> MGSSLMTEHKKRIDPVGAMLESKLLEAEFSPAVAAKLAALSQHYTPAELVRALPQSLANMLDNQGDDIVRQGGVVALVGPTGVGKTTSLAKLAARFAAHHGPEQVALITTDHYRIGAYEQLATYGKIMGCPVKQAHDLNELEQILYQFRNRKLVLIDTAGMGQRDMRLYQQLDNLTANSRIPIRSYLVLSATGQRRVLQDAVNHFKRIPLSGAVLTKLDESVSLAGALSVLIQSGLPLSYVTDGQRVPEDMKVADTLMLAQQALATLDSTEQQSLQDTAWSDNMACAFEHHHHHH

The GTPase FlhF, a signal recognition particle (SRP)-type enzyme, is pivotal for spatial–numerical control and bacterial flagella assembly across diverse species, including pathogens. FlhF, together with SRP54 (or Ffh) and FtsY, belongs to an evolutionarily conserved protein family with only three members: the signal recognition particle (SRP) GTPases. The three SRP GTPases share a conserved NG domain, with the N domain comprising an α-helical bundle and the G domain being a GTPase with an α–β–α insertion termed the I-box. The GTPase activity of the FlhF homodimer and its dissociation into a GDP-bound monomer is stimulated by the protein FlhG, which serves as numerical regulator of flagella biosynthesis.

In this report, we present the biochemical and structural analysis of a GDP-bound monomer of FlhF from the polar-flagellated bacterium Shewanella putrefaciens CN32. Expression of NG-FlhF yielded approximately 40 mg per litre of culture (equivalent to 8 g of cells) and protein purification followed standard protocols described previously. Analytical size-exclusion chromatography (SEC) revealed the presence of a monomer. Amino-acid residues 183–437 of NG-FlhF could be unambiguously assigned into the electron-density map and represent almost all of the residues of the protein construct employed in this study. The structure of NG-FlhF reveals that of a classical NG domain of the SRP-GTPase family. The GDP is coordinated by residues of the G1, G4 and G5 elements, which are conserved among the SRP GTPase family. In the GDP-bound state of FlhF, the guanine base of the nucleotide is coordinated by Asp388 and Glu389 of the G4 element. The α- and β-phosphates of GDP are coordinated by Lys254, Thr255 and Thr256 of the G1 element. Density for a magnesium ion was not present within the active site of NG-FlhF. Most prominently, Arg283 within the G2 loop is properly ordered in our structure, coordinating the β-phosphate of the GDP. The binding of GDP introduces a rotation of 20–40° of the helices of the bundle in relation to its center.>[2x]ELDGDQMISHRELWAKIANSINDINEQYLKVYEHAVSSYTQMYQDFSAVLSSLAGWISPGGNDGNSVKLQVNSLKKALEELKEKYKDKPLYPANNTVSQEQANKWLTELGGTIGKVSQKNGGYVVSINMTPIDNMLKSLDNLGGNGEVVLDNAKYQAWNAGFSAEDETMKNNLQTLVQKYSNANSIFDNLVKVLSSTIS

Like many Gram-negative pathogens, Shigella rely on their type three secretion system (T3SS) to inject effector proteins into eukaryotic host cells, driving both cellular invasion and evasion of host immune responses. Studies in Shigella have demonstrated that bile salts found in the small intestine (e.g., deoxycholate (DOC)) interact directly with the injectisome tip complex protein invasion plasmid antigen D (IpaD) to support interaction with the hydrophobic translocator protein IpaB and its stable recruitment to the maturing tip complex. In Shigella, IpaD resides at the extracellular tip of the injectisome where it functions as a “gatekeeper” that prevents unwanted protein secretion (leakage) through the injectisome prior to requisite activation events. Here, we uncover critical mechanistic details of the Shigella-specific DOC signaling process by describing the role of a π-helix secondary structure element within the T3SS tip protein invasion plasmid antigen D (IpaD).

X-ray crystal structures of DOC-bound IpaDWT and DOC-bound IpaDΔQ148 were critical for resolving this apparent conflict by providing the first molecular insight into the role of IpaD’s π-helix in the DOC-mediated Shigella virulence enhancement pathway. More specifically, comparing these structures shows that eliminating the π-helix does not eliminate DOC binding, but instead causes the single binding site for DOC to migrate approximately 10 Å, now docking in the cleft between the two central helices where the elimination of the π-helix occurred. A closer look at the side chains located within 4.5 Å of the bound DOCs shows that while some polar and charged side chains such as lysine 137 and serine 141 in the native binding site and aspartate 144 and serine 141 in the modified site of the π-helix deletion construct are in the vicinity of the DOC binding sites, they are oriented away from the bound DOC and do not appear to contribute to binding through electrostatic interactions. Instead, both DOC interactions are driven nearly exclusively through hydrophobic interactions. Furthermore, the π-helix backbone atoms in the WT structure also occlude the distal end of the mutant DOC binding site.The Z (Glu342Lys) mutation causes α1-antitrypsin, the major circulating human antiprotease, to misfold and self-associate into polymers within the endoplasmic reticulum of hepatocytes, with toxic gain-of-function effects. The concomitant deficiency of circulating protein renders lung tissue vulnerable to destructive and proinflammatory effects of neutrophil elastase, that is the physiological target of α1-antitrypsin, and hence a clinical association with early-onset emphysema. It proceeds from a metastable native state, via an unstable monomeric intermediate state that is polymerogenic (M*), to a hyperstable polymer assembly. All three methods were used for the detailed characterization of the interaction of α1-antitrypsin with the reactive loop analogue tetrapeptide Thr-Thr-Ala-Ile (TTAI), the most promising polymerization-blocking peptide developed to date.

The binding of two copies of TTAI was associated with a decrease in the normalized value for residues between helix D and s2A and an increase for residues between helix I and s5A around the lower peptide insertion site. Away from β-sheet A, RMSD comparisons of the crystallographic positions of backbone and side-chain atoms indicated minimal differences. Comparison of the similarly high-resolution crystal structures of native (1.8 Å; PDB ID: 3NE447) and TTAI-saturated α1-antitrypsin shows that only β-sheet A undergoes substantial structural change. However, in solution, TTAI binding significantly perturbs the backbone chemical shifts for the majority of residues in the protein, with the exception of those within β-sheet C, which are relatively unaffected. This indicates that, in addition to the clear structural changes in β-sheet A seen in the crystal structure, TTAI binding in solution induces subtle but detectable changes throughout the rest of the protein. Taken together, these data strongly support the binding of two TTAI peptides in the upper and lower parts of the s4A site in α1-antitrypsin, with binding of the first peptide facilitating patency of the rest of the site for the second. Integration of these findings with B-factor analysis of the high-resolution X-ray crystallographic structural data supports a model in which TTAI binds sequentially within s4A. In this model, the first TTAI peptide anneals to the more labile “breach” region at the base of the reactive loop between strands 3 and 5 of β-sheet A (s3A, s5A). The binding of two TTAI molecules stabilizes the protein in a ternary complex by favoring the population of compact conformers relative to more extended states such as those previously defined by IM-MS as polymerogenic intermediates.

> MRGSHHHHHHTDPQGDAAQKTDTSHHDQDHPTFNKITPNLAEFAFSLYRQLAHQSNSTNIFFSPVSIATAFAMLSLGTKADTHDEILEGLNFNLTEIPEAQIHEGFQELLRTLNQPDSQLQLTTGNGLFLSEGLKLVDKFLEDVKKLYHSEAFTVNFGDTEEAKKQINDYVEKGTQGKIVDLVKELDRDTVFALVNYIFFKGKWERPFEVKDTEEEDFHVDQVTTVKVPMMKRLGMFNIQHCKKLSSWVLLMKYLGNATAIFFLPDEGKLQHLENELTHDIITKFLENEDRRSASLHLPKLSITGTYDLKSVLGQLGITKVFSNGADLSGVTEEAPLKLSKAVHKAVLTIDEKGTEAAGAMFLEAIPMSIPPEVKFNKPFVFLMIEQNTKSPLFMGKVVNPTQK>GPMPQLTLDKTDIKILQVLQENGRLTNVELSERVALS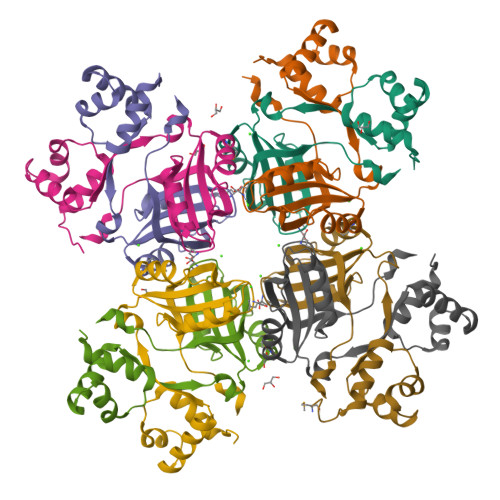PSPCLRRLKQLEDAGIVRQYAALLSPESVNLGLQAFIRVSIRKAKDAREDFAASVRKWPEVLSCFALTGETDYLLQAFFTDMNAFSHFVLDTLLSHHGVQDAQSSFVLKEIKHTTSLPLNHLLKE[8x]>MASEALTMIVNLLRSQRPLQEPTVEQMRAGLEAMAQMSPLPADVELTTVDAGGVPGAWVRVPESDPDRVVLYLHGGGYVIGSIRTHRDLAQRIARAARCRVLLIDYRLAPEHPHPAAVEDSTRAYRWLLETGSDPKRMAIAGDAAGGGLTVATLVALRDAGVPLPAAAVCLS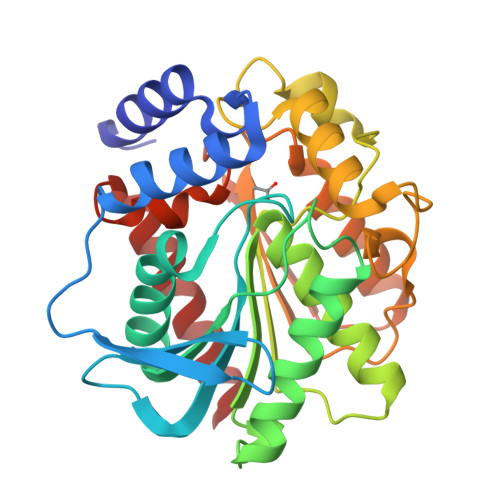PWVDLEGIGESMTTKAAVDPMVQREPLLRMASMYLAGQDPRTPLAAPLYADLRGLPPLLIQVGTAETLLDDSVRLAERARAAGVQVTLEPWEDMIHVWQAFAAMLPEGQQAIERIGEFLRQHWQ[2x]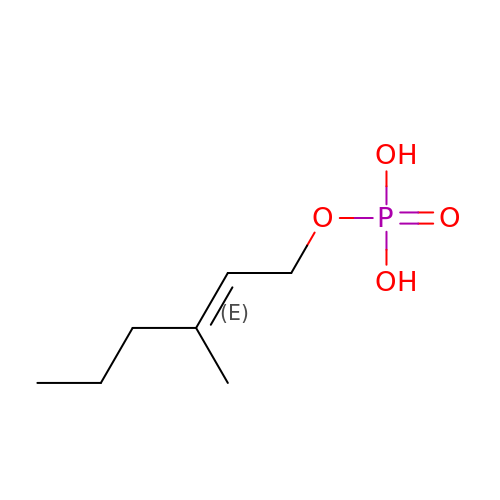[(~{E})-3-methylhex-2-enyl] dihydrogen phosphate | C7 H15 O4 P | QFTXOINSFIOLQI-FNORWQNLSA-N>[8x]SVDHGFLVTRHSQTTDDPQCPPGTKILYHGYSLLYVQGNERAHGQDLGTAGSCLRKFSTMPFLFCNINNVCNFASRNDYSYWLSTPEPMPMSMAPITGENIRPFISRCAVCEAPAMVMAVHSQTIQIPQCPTGWSSLWIG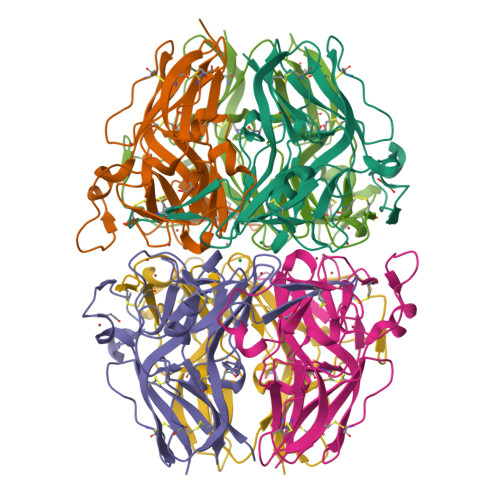YSFVMHTSAGAEGSGQALASPGSCLEEFRSAPFIECHGRGTCNYYANAYSFWLATIERSEMFKKPTPSTLKAGELRTHVSRCQVCMRRT;>[4x]ISIGYLLVKHSQTDQEPMCPVGMNKLWSGYSLLYFEGQEKAHNQDLGLAGSCLARFSTMPFLYCNPGDVCYYASRNDKSYWLSTTAPLPMMPVAEEDIRPYISRCSVCEAPAVAIAVHSQDVSIPHCPAGWRSLWIGYSFLMHTAAGDEGGGQSLVSPGSCLEDFRATPFIECNGARGTCHYYANKYSFWLTTIPEQSFQGTPSADTLKAGLIRTHISRCQVCMKNL> SGGALDLKTQVQ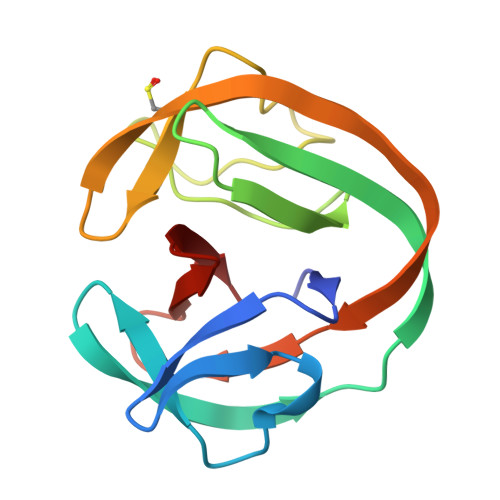TPQGMKEISNIQVGDLVLSNTGYNEVLNVFPKSKKKSYKITLEDGKEIICSEEHLWPTQTGEMNISGGLKEGMCLYVKEMMLKKILKIEELDERELICIEVSGNHLFYANDILTHN BENZENE-1,2,4,5-TETROL | C6 H6 O4 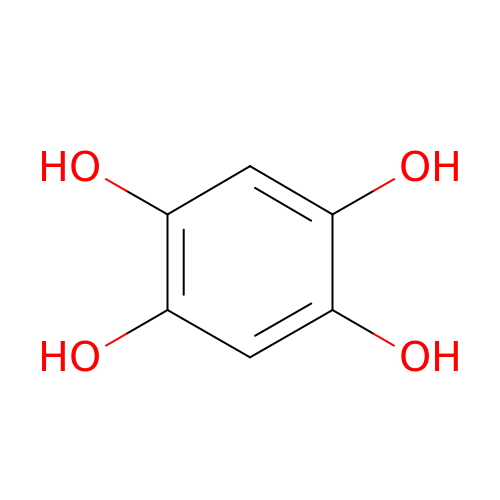| UYQMSQMCIYSXOW-UHFFFAOYSA-N> 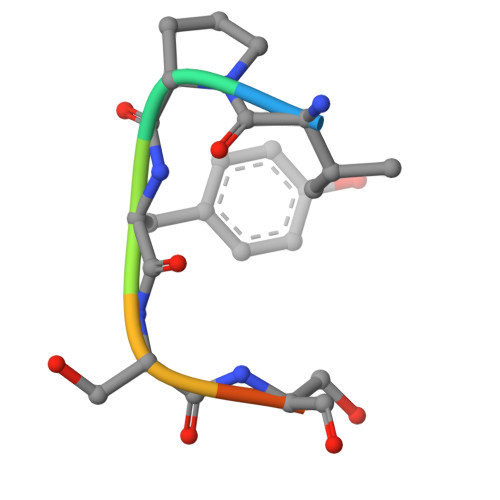VPYSSAQ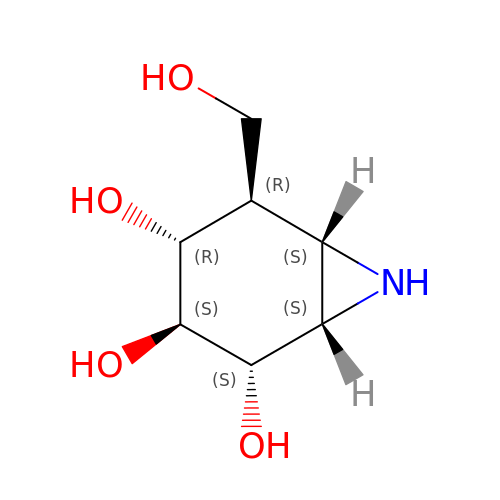(1~{S},2~{S},3~{S},4~{R},5~{R},6~{S})-5-(hydroxymethyl)-7-azabicyclo[4.1.0]heptane-2,3,4-triol | C7 H13 N O4 | GPIFFOGPRPKRHS-GESKJZQWSA-N> MLYTRRLMTTGGSATADGAVSYSKGSYHIVPKKYTVGKRIAVRSYLDRNRTELSDRTYMPQKAWFEPYTPKKFDMEHQRISHNFYNLETKLIWTAFDTPELIGILLHDETIKGAPHLYDAEFLESAVHWTRESRYWRCIGITKPFYNKTTLRAQCWHDRGLQVGTLVFSQAMRDALMDLERAVRRKELGLEPNYVWDRWGPVGFIDGARTDHLPRFAHNPYVDPD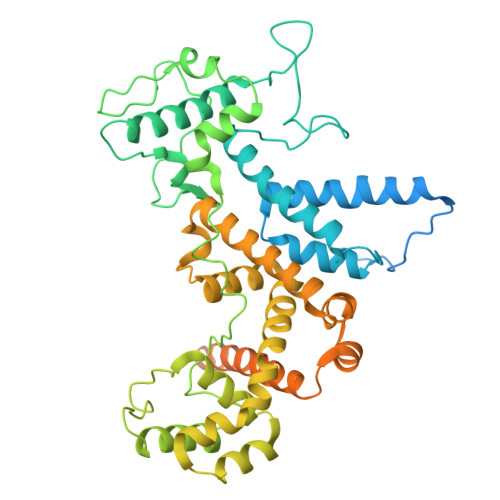GVEVTEVDIAPFNTHEQIKERYGAFIDPDLRPFEGVFRSSSSSSSSSSSSSSSSSSSSSSSSSSSSSSSSSSSSSSSSSSSSSSSSSSSSSSSSSSSSSSSSSSSSSSSSSSSSSSSSCDEKVEALRLMENTRHDAARVRTFYEEKCGFSDFMRTPDKVITAAVLCYLQELQRICTETDWGKPLARCLTDLERVNVMGKDAFLVYRHIEDAILDKKRRVWATRFAGEANEESTLDYLLENFGRRTEQTRNVGTTGTEFDREQEPIGRQVQRRVLDSDKASKLAEVRQKRGKMWSNKKSVFDSLHQKQLQNVTYGVH>GSKQNQKSVNKHDKEALYRYYTGKTMEMKNISALKHGKNNLRFKFRGIKIQVLLPGNDKSKFQQRSYEGLDVFFVQEKRDKHDIFYTVGGVIQNNKTSGVVSAPILNISKEKGEDAFVKGYPYYIK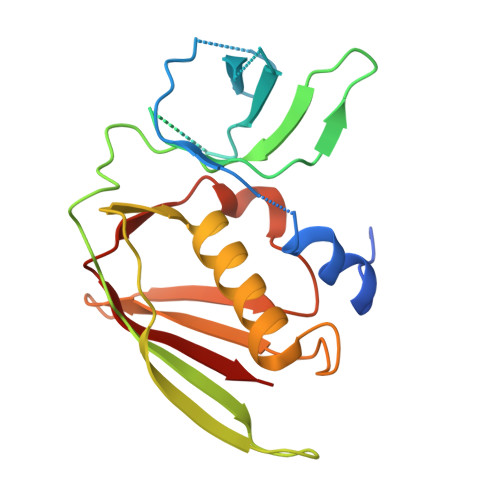KEKITLKELDYKLRKHLIEKYGLYKTISKDGRVKISLKDGSFYNLDLRSKLKFKYMGEVIESKQIKDIEVNLK[2x]> GKTITGVFNSFNSLTWSNAATYNYKGPGTPTWNAVLGWSLDGTSASPGDTFTLNMPCVFKFTTSQTSVDLTAHGVKYATCQFQAGEEFMTFSTLTCTVSNTLTPSIKALGTVTLPLAFNVGGTGSSVDLEDSKCFTAGTNTVTFNDGGKKISINVDFERSNVDPKGYLTDSRVIPSLNKVSTLFVAPQCANGYTSGTMGFANTYGDVQIDCSNIHVGITKGLNDWNYPVSSESFSYTKTCSSNGIFITYKNVPAGYRPFVDAYISATDVNSYTLSYANEYTCAGGYWQRAPFTLRWTGYR;> TTTTTTT

Cell surface glycoproteins in the C. albicans Als family (Als1–Als7 and Als9) are most commonly associated with adhesion of the fungus to host cells, as well as more complex interactions such as invasion and biofilm formation, for which adhesion is a prerequisite (7–9). Als proteins are one of the most widely studied C. albicans virulence attributes; deletion of ALS3 produces the greatest reduction in adhesive function. The N-terminal domain of Als proteins (NT-Als)4 was implicated in adhesive function, prompting work to solve its structure. An invariant Lys (Lys-59) at the end of the PBC recognizes the carboxyl group at the C terminus of a peptide ligand, allowing the remaining peptide backbone to associate in parallel orientation with β-strand G2.

Removal of the C-terminal AFR to form sNT-Als3 (amino acids 1–302) resulted in a folded protein that was monomeric in solution, with excellent dispersion of amide resonances. sNT-Als3shorter version of NT-Als3 that excludes the C-terminal AFR. The crystal structure of sNT-Als3 (amino acids 1–302) in complex with the model peptide hepta-Thr showed that removal of the C-terminal AFR did not affect the formation of a fully functional PBC. Notably, the side chain amine of Lys-59 formed a salt bridge with the C-terminal carboxylate of the hepta-Thr ligand, and at least 12 hydrogen bonds between the peptide in extended conformation and this binding cavity were connected via water molecules, resembling the mode of interaction observed in the structure of the NT-Als9-2·Fg-γ complex. In the residues comprising the immunoglobulin “core” (amino acids 1–299 of the mature protein), this construct had the same overall structure as NT-Als3-pbc, with a r.m.s.d. of 0.9 Å for 296 Cα carbons (DaliLite). When hepta-Thr was bound in the PBC, the Tyr-301 side chain was exposed to the solvent and did not contact Lys-59, possibly from electrostatic repulsion experienced by unpaired charges of the carboxyl group and side chain of Arg-302 at the C terminus. The observation that sNT-Als3 bound hepta-Thr was confirmed in solution by ITC. In the structure of different NT-Als·ligand complexes, several water molecules anchor polypeptides with different C-terminal sequences in the PBC.> MGNNVVVLGTQWGDEGKGKIVDLLTERAKYVVRYQGGHNAGHTLVINGEKTVLHLIPSGILRENVTSIIGNGVVLSPAALMKEMKELEDRGIPVRERLLLSEACPLILDYHVALDNAREKARGAKAIGTTGRGIGPAYEDKVARRGLRVGDLFDKETFAEKLKEVMEYHNFQLVNYYKAEAVDYQKVLDDTMAVADILTSMVVDVSDLLDQARQRGDFVMFEGAQGTLLDIDHGTYPYVTSSNTTAGGVATGSGLGPRYVDYVLGILKAYSTRVGAGPFPTELFDETGEFLCKQGNEFGATTGRRRRTGWLDTVAVRRAVQLNSLSGFCLTKLDVLD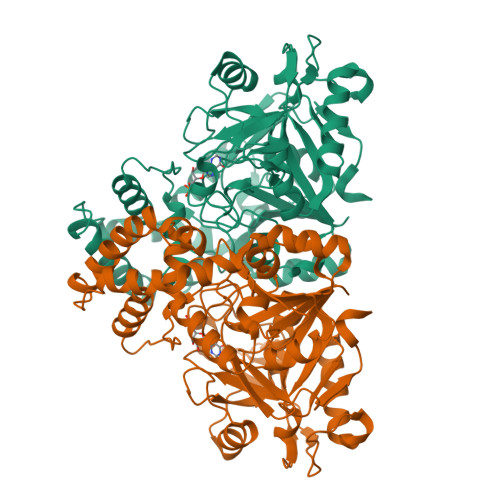GLKEVKLCVAYRMPDGREVTTTPLAADDWKGVEPIYETMPGWSESTFGVKDRSGLPQAALNYIKRIEELTGVPIDIISTGPDRTETMILRDPFDA(1R)-N-(prop-2-en-1-yl)-2,3-dihydro-1H-inden-1-amine | C12 H15 N | 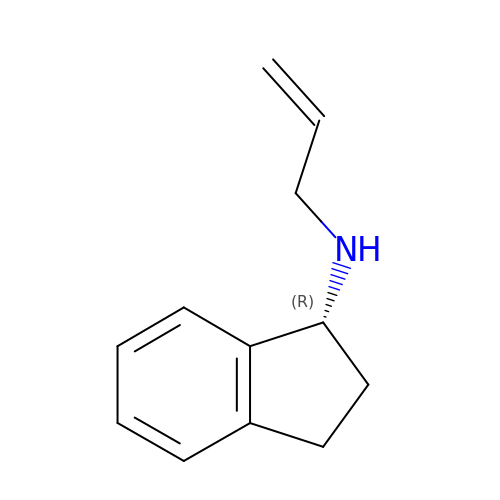RPAZWTZFMPXUKS-GFCCVEGCSA-N> SLGAKPFGEKKFIEIKGRRMAYIDEGTGDPILFQHGNPTSSYLWRNIMPHCAGLGRLIACDLIGMGDSDKLDPSGPERYAYAEHRDYLDALWEALDLGDRVVLVVHDWGSALGFDWARRHRERVQGIAYMEAIAMPIEWADFPEQDRDLFQAFRSQAGEELVLQDNVFVEQVLPGLILRPLSEAEMAAYREPFLAAGEARRPTLSWPRQIPIAGTPADVVAIARDYAGWLSESPIPKLFINAEPGALTTGRMRDFCRTWPNQTEITVAGAHFIQEDSPDEIGAA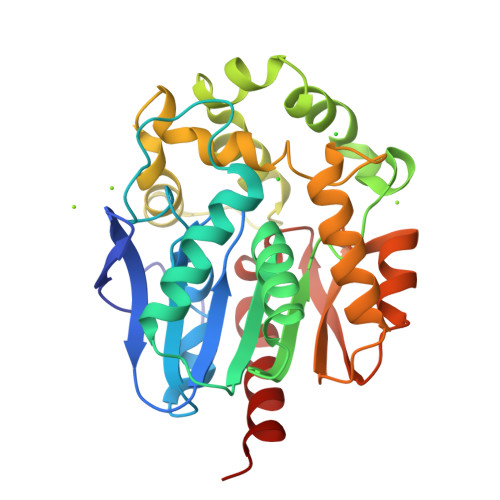IAAFVRRLRPA> MLEKLNNINFNNISNNLNLGIEVGREIQNASWIKSPFFSITGTGADRGVRLFSVASQQPFRPRIKAQLSGSGVSGNTDFEANYDNLEILSQTIYPDAFGNSLRSKIKAYSELERIDFIKESVDSLTTWMNEERDKRIVASLTNDFTNYLYTQTMNVATIRKAIFHARNGLKGDNSKAFPIKPIRATMQSVGNVMVQNTSYIILLDSYQANQLKADSEFKELRKLYAFAGEDKGMLYSGLLGVIDNCPVIDAGVWNKFNVGMPNSSISDSDFMRYLNKANVSSIVTPRQFKEKLNQEKDEKKRSINKEISIGCLIGASAVLLAGSKETRFYIDETVDAGRKSLVGVDCLLGVSKARYQSTDGVVTPYDNQDYAVIGLVSD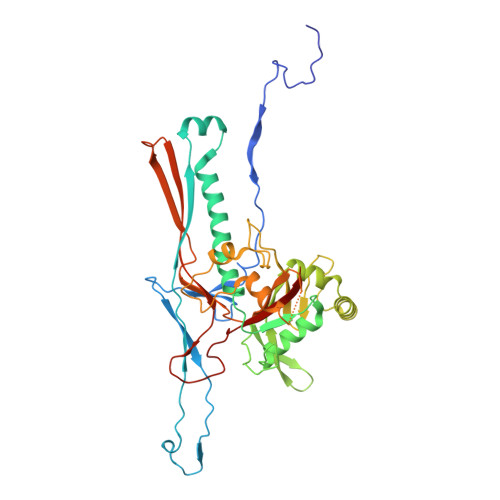ME>[2x]APPPYAKQVERDFLTCLTKDIPPRQLYAKSSPAYASVWSSTVRNIKFLSDKTVKPLYIITPTNASHIQAAVVCGRRHGMRIRVRSGGHDYEGLSYRSEKPEPFAVVDMNKMRAVSIDGKAATAWVDSGAQLGDLYYGIAKA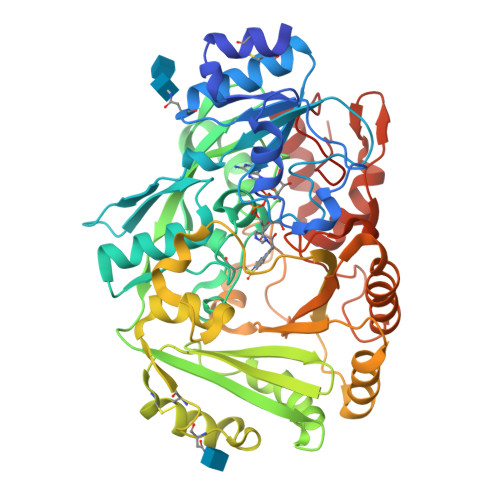SPKLGFPAGVCTTIGVGGHFSGGGFGMLLRKYGTAADNVIDAKVVDAQGRLLDRKAMGEDHFWAIRGGGGESFGIVASWQVKLLPVPPKVTVFQVHKGIKEGAIDLVTKWQTVAPALPDDLMIRIMAMGQGAMFEALYLGTCKDLVLLMTARFPELGMNATHCKEMTWIESVPYIPMGPKGTVRDLLNRTSNIKAFGKYKSDYVLEPIPKSDWEKIFTWLVKPGAGVMIMDPYGGGIASVPESATPFPRRSGVLFNIQYVVYWFGEGAAALPTQWTRDIYDFMTPYVSKNPRQAYVNYRDLDLGVNQVVGNVSTYASGKVWGEKYFKGNFERLARTKGKIDPEDYFRNEQSIPPLL> RGEEEQWAREIGAQL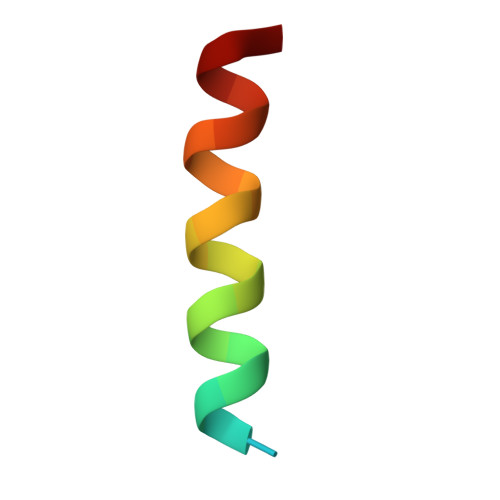RRMADDLN> MGANASALEKEIGPEQFPVNEHYFGLVNFGNTCYCNSVLQALYFCRPFREKVLAYKSQPRKKESLLTCLADLFHSIATQKKKVGVIPPKKFITRLRKENELFDNYMQQDAHEFLNYLLNTIADILQEERKQEKQNGRLPNGNIDNENNNSTPDPTWVHEIFQGTLTNETRCLTCETISSKDEDFLDLS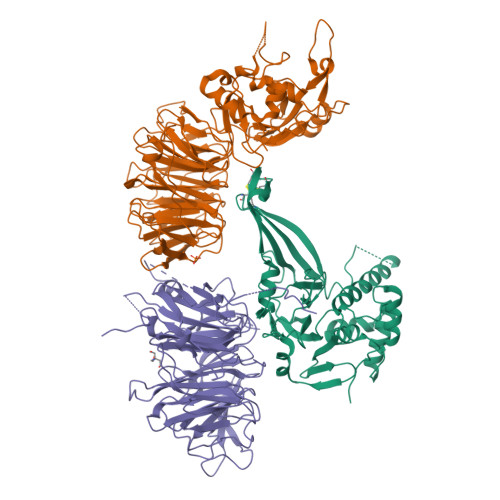VDVEQNTSITHCLRGFSNTETLCSEYKYYCEECRSKQEAHKRMKVKKLPMILALHLKRFKYMDQLHRYTKLSYRVVFPLELRLFNTSGDATNPDRMYDLVAVVVHCGSGPNRGHYIAIVKSHDFWLLFDDDIVEKIDAQAIEEFYGLTSDISKNSESGYILFYQSRD;> MAAHHRQNTAGRRKVQVSYVIRDEVEKYNRNGVNALQLDPALNRLFTAGRDSIIRIWSVNQHKQDPYIASMEHHTDWVNDIVLCCNGKTLISASSDTTVKVWNAHKGFCMSTLRTHKDYVKALAYAKDKELVASAGLDRQIFLWDVNTLTALTASNNTVTTSSLSGNKDSIYSLAMNQLGTIIVSGSTEKVLRVWDPRTCAKLMKLKGHTDNVKALLLNRDGTQCLSGSSDGTIRLWSLGQQRCIATYRVHDEGVWALQVNDAFTHVYSGGRDRKIYCTDLRNPDIRVLICEEKAPVLKMELDRSADPPPAIWVATTKSTVNKWTLKGIHNFRASGDYDNDCTNPITPLCTQPDQVIKGGASIIQCHILNDKRHILTKDTNNNVAYWDVLKACKVEDLGKVDFEDEIKKRFKMVYVPNWFSVDLKTGMLTITLDESDCFAAWVSAKDAGFSSPDGSDPKLNLGGLLLQALLEYWPRTHVNPMDEEENEVNHVNGEQENRVQKGNGYFQVPPHTPVIFGEAGGRTLFRLLCRDSGGETESMLLNETVPQWVIDITVDKNMPKFN;> MATEGGGKEMNEIKTQFTTREGLYKLLPHSEYSRPNRVPFNSQGSNPVRVSFVNLNDQSGNGDRLCFNVGRELYFYIYKGVRKAADLSKPIDKRIYKGTQPTCHDFNHLTATAESVSLLVGFSAGQVQLIDPIKKETSKLFNEERLIDKSRVTCVKWVPGSESLFLVAHSSGNMYLYNVEHTCGTTAPHYQLLKQGESFAVHTCKSKSTRNPLLKWTVGEGALNEFAFSPDGKFLACVSQDGFLRVFNFDSVELHGTMKSYFGGLLCVCWSPDGKYIVTGGEDDLVTVWSFVDCRVIARGHGHKSWVSVVAFDPYTTSVEEGDPMEFSGSDEDFQDLLHFGRDRANSTQSRLSKRNSTDSRPVSVTYRFGSVGQDTQLCLWDLTEDILFPHQPLSRARTHTNVMNATSPPAGSNGNSVTTPGNSVPPPLPRSNSLPHSAVSNAGSKSSVMDGAIASGVSKFATLSLHDRKERHHEKDHKRNHSMGHISSKSSDKLNLVTKTKTDPAKTLGTPLCPRMEDVPLLEPLICKKIAHERLTVLIFLEDCIVTACQEGFICTWGRPGKVVSFNP6,7,8,9-TETRAHYDRO-4-HYDROXY-3-(1-PHENYLPROPYL)CYCLOHEPTA[B]PYRAN-2-ONE 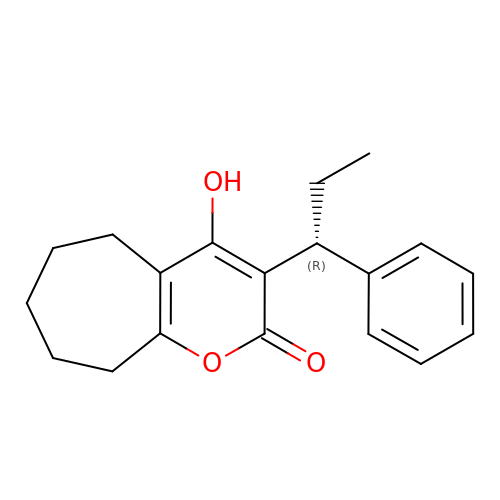| C19 H22 O3 | YKJXQZGJGDTEOC-AWEZNQCLSA-N>MRLTDVDLTVGEETREYAVSEQQGTLFR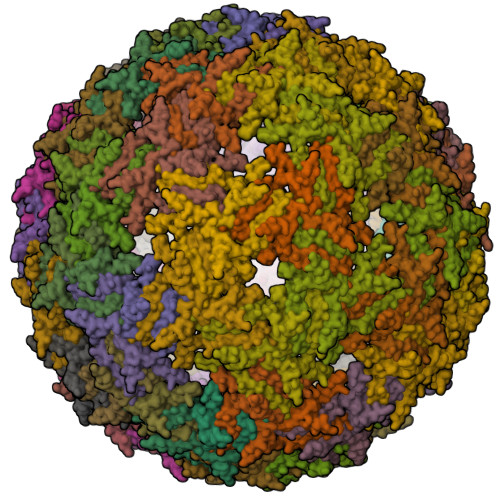FVDKSGTVANNTGVFSLEQRFGAANSNRKVTMLLTDPVVVKDASGADMTIKANASVTFSLPKTYPNEHITKLRQTLIAWLGQQCVSDPVDSGLNNY[180x]> DTAIEKRLASLLT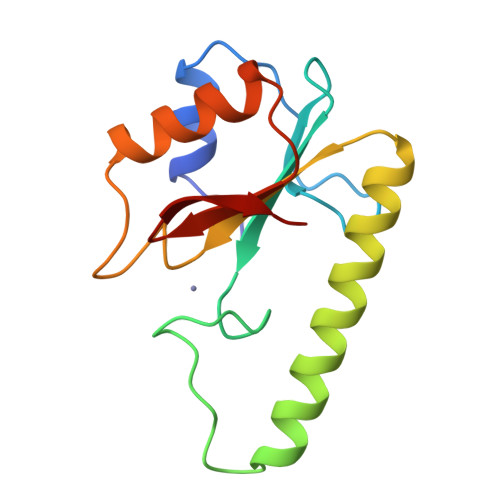GQGLAFRVQDASLPGRPDFVVDEYRCVIFTHGCFWHHHHCYLFKVPATRTEFWLEKIGKNVERDRRDISRLQELGWRVLIVWECALRGREKLTDEALTERLEEWICGEGASAQIDTQGIHLLA> GGAUCUUCGGGGCAGGGUGAAAUUCCCGAC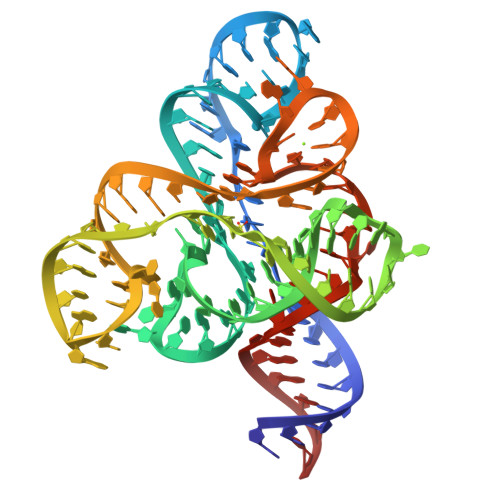CGGUGGUAUAGUCCACGAAAGUAUUUGCUUUGAUUUGGUGAAAUUCCAAAACCGACAGUAGAGUCUGGAUGAGAGAAGAUUC>MGAQVSTQKTGAHETGLNASGNSIIHYTNMNYYKDSASNSANRQEFAQDPGKFTEPVKDIMIKSMPALNSPSAEECGYSDRVRSITLGNSTITTQECANVVVGYGTWPTYLRDEEATAEDQPTQPDVATCRFYTLESVMWQQSSPGWWWKFPDALSNMGLFGQNMQYHYLGRAGYTLHVQCNASKFHQGCLLVVCVPEAEMGCATIANKPDQKSLSNGETANVFDSQNTSGQTAVQANVINAGMGIGVGNLTIFPHQWINLRTNNSATIVMPYVNSVPMDNMFRHNNFTLMIIPFAPLSYSTGATTYVPITVTVAPMCAEYNGLRLAGRQGLPTMLTPGSNQFLTSDDFQSPSAMPQFDVTPEMAIPGQVNNLMEIAEVDSVVPVNNTEGKVMSIEAYQIPVQSNSTNGSQVFGFPLIPGASSVLNRTLLGEILNYYTHWSGSIKLTFMFCGSAMATGKFLLAYSPPGAGAPTTRKEAMLGTHVIWDVGLQSSCVLCIPWISQTHYRYVVMDEYTAGGYITCWYQTNIVVPADTQSDCKILCFVSACNDFSVRMLKDTPFIKQDSFFQGPPGEAIERAIARVADTISSGPVNSESIPALTAAETGHTSQVVPADTMQTRHVKNYHSRSESTVENFLCRSACVYYTTYKNHGTDGDNFAQWVINTRQVAQLRRKLEMFTYARFDLELTFVITSSQEQSTIKGQDSPVLTHQIMYVPPGGPVPTKINSYSWQTSTNPSVFWTEGSAPPRISIPFISIGNAYSMFYDGWARFDKQGTYGINTLNNMGTLYMRHVNDGSPGPIVSTVRIYFKPKHVKTWVPRPPRLCQYQKAGNVNFEPSGVTEGRTEITAMQTT[3x]

Enteroviruses are nonenveloped positive single-stranded (ss) RNA viruses and are major causative agents of waterborne diseases. Coxsackievirus B5 (CVB5) is a genotype of the Enterovirus genus, which is frequently detected in clinical and wastewater surveillance. Here, we employed a reverse genetic system for CVB5 and assessed how different amino acid substitutions in capsid proteins affects the virus’ sensitivity to free chlorine and heat. To elucidate the mechanism behind reduced heat sensitivity of the CVB5F.cas.genogroupB mutant, we subjected it to analysis by cryoEM.

We applied a combination of 2D and 3D classification steps in cryoSPARC package to separate the particles corresponding to mature virions (F), intermediate-altered state (A), and empty viral capsids (E). These conformational states are commonly resolved in cryoEM analyses of enteroviruses, with A and E corresponding to the expanded viral particles with or without the internal viral components (nonstructural proteins and genetic material). The resulting EM density maps were at 3.6, 2.7, and 2.6 Å global resolution for the capsid-corresponding part of particles F, A, and E, respectively, thus allowing building of atomic models of each state. The two amino acid substitutions causing the largest perturbation in relative heat sensitivity, VP1.D276E, and VP1.T279A, are located at the C-terminus of VP1. These two residues interact with each other and contribute to the external part of the VP1:VP3 interface, both through direct contact and indirectly by stabilization of the local loop region comprising residues VP1.E272-T282. Consistently, this region in VP1 undergoes partial restructuring in intermediate-altered (A) and empty particle (E) states, with alanine at VP1.279 facing toward the hydrophobic pocket in VP3 assembled by residues VP3.P86, VP3.A141 and VP3.Y189. Although the C-terminus of VP1 is flexible in different enterovirus structures, the resulting conformation in A and E particles of CVB5F.cas.genogroupB is distinct from the previously published reconstruction of CVB5-A and E particles having the original VP1.D276/VP1.T279 pairing (Figure S3 and the previous study64), supporting that VP1.D276E and VP1.T279A mutations may affect the assembly and local dynamics of the VP1:VP3 interface. Several other areas in particle A and E states of CVB5F.cas.genogroupB also exhibit different conformations and/or greater flexibility compared with corresponding CVB5 structures from the PDB. Most prominent changes were in the N-terminal region of VP1 (VP1.Q49-S60), VP2 (VP2.L42-Q52), and VP3 (I168–V181). Altogether, based on structural analysis of the CVB5F.cas.genogroupB we propose that mutations conferring greater tolerance to thermal inactivation by perturbing local molecular interactions which may lead to improved stability of infectious virions (F) and altered conformations of uncoating intermediates (e.g., particles A and E).>PKLVLVRHGQSEWNEKNLFTGWVDVKLSAKGQQEAARAGELLKEKKVYPDVLYTSKLSRAIQTANIALEKADRLWIPVNRSWRLNERHYGDLQGKDKAETLKKFGEEKFNTYRRSFDVPPPPIDASSPFSQKGDERYKYVDPNVLPETESLALVIDRLLPYWQDVIAKDLLSGKTVMIAAHGNSLRG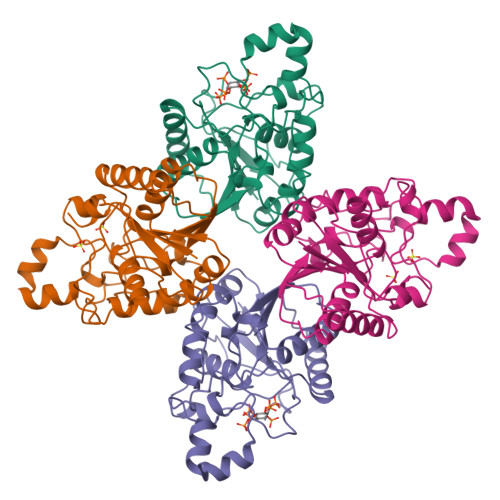LVKHLEGISDADIAKLNIPTGIPLVFELDENLKPSKPSYYLDPEAAAAGAAAVANQGKK[4x]>[4x]CPRFLKVKNWETEVVLTDTLHLKSTLETGCTEYICMGSIMHPSQHARRPEDVATKDQLFPLAKEFIDQYYSS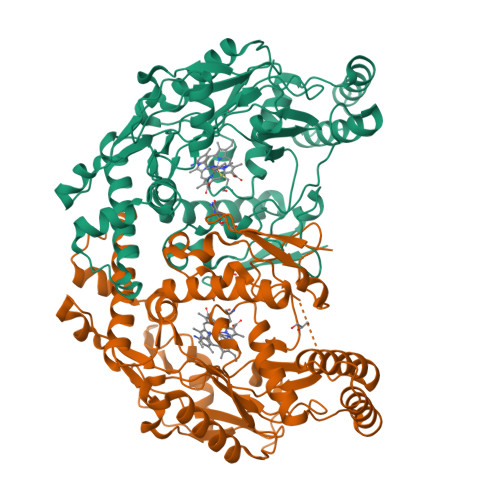IKRFGSKAHMERLEEVNKEIDTTSTYQLKDTELIYGAKHAWRNASRCVGRIQWSKLQVFDARDCTTAHGMFNYICNHVKYATNKGNLRSAITIFPQRTDGKHDFRVWNSQLIRYAGYKQPDGSTLGDPANVQFTEICIQQGWKPPRGRFDVLPLLLQANGNDPELFQIPPELVLEVPIRHPKFEWFKDLGLKWYGLPAVSNMLLEIGGLEFSACPFSGWYMGTEIGVRDYCDNSRYNILEEVAKKMNLDMRKTSSLWKDQALVEINIAVLYSFQSDKVTIVDHHSATESFIKHMENEYRCRGGCPADWVWIVPPMSGSITPVFHQEMLNYRLTPSFEYQPDPWNTHVWKLV> GVALGATRVIYPAGQKQVQLAVTNNDENSTYLIQSWVENADGVKDGRFIVTPPLFAMKGKKENTLRILDATNNQLPQDRESLFWMNVKAIPSMDKSKLTENTLQLAIISRIKLYYRPAKLALPPDQAAEKLRFRRSANSLTLINPTPYYLTVTELNAGTRVLENALVPPMGESTVKLPSDAGSNITYRTINDYGALTPKMTGVMEHHHHHH;> DLYFNPRFLADDPQAVADLSRFENGQELPPGTYRVDIYLNNGYMATRDVTFNTGDSEQGIVPCLTRAQLASMGLNTASVAGMNLLADDACVPLT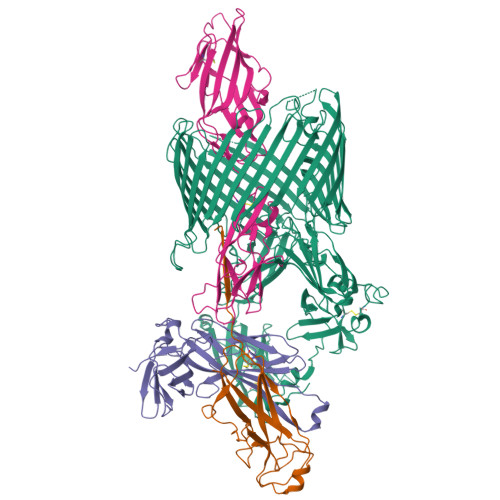TMVQDATAHLDVGQQRLNLTIPQAFMSNRARGYIPPELWDPGINAGLLNYNFSGNSVQNRIGGNSHYAYLNLQSGLNIGAWRLRDNTTWSYNSSDRSSGSKNKWQHINTWLERDIIPLRSRLTLGDGYTQGDIFDGINFRGAQLASDDNMLPDSQRGFAPVIHGIARGTAQVTIKQNGYDIYNSTVPPGPFTINDIYAAGNSGDLQVTIKEADGSTQIFTVPYSSVPLLQREGHTRYSITAGEYRSGNAQQEKPRFFQSTLLHGLPAGWTIYGGTQLADRYRAFNFGIGKNMGALGALSVDMTQANSTLPDDSQHDGQSVRFLYNKSLNESGTNIQLVGYRYSTSGYFNFADTTYSRMNGYNIETQDGVIQVKPKFTDYYNLAYNKRGKLQLTVTQQLGRTSTLYLSGSHQTYWGTSNVDEQFQAGLNTAFEDINWTLSYSLTKNAWQKGRDQMLALNVNIPFSHWLRSDSKSQWRHASASYSMSHDLNGRMTNLAGVYGTLLEDNNLSYSVQTGYAGGGDGNSGSTGYATLNYRGGYGNANIGYSHSDDIKQLYYGVSGGVLAHANGVTLGQPLNDTVVLVKAPGAKDAKVENQTGVRTDWRGYAVLPYATEYRENRVALDTNTLADNVDLDNAVANVVPTRGAIVRAEFKARVGIKLLMTLTHNNKPLPFGAMVTSESSQSSGIVADNGQVYLSGMPLAGKVQVKWGEEENAHCVANYQLPPESQQQLLTQLSAECR;> ADSTITIRGYVRDNGCSVAAESTNFTVDLMENAAKQFNNIGATTPVVPFRILLSPCGNAVSAVKVGFTGVADSHNANLLALENTVSAASGLGIQLLNEQQNQIPLNAPSSALSWTTLTPGKPNTLNFYARLMATQVPVTAGHINATATFTLEYQ;> FACKTANGTAIPIGGGSANVYVNLAPVVNVGQNLVVDLSTQIFCHNDYPETITDYVTLQRGSAYGGVLSNFSGTVKYSGSSYPFPTTSETPRVVYNSRTDKPWPVALYLTPVSSAGGVAIKAGSLIAVLILRQTNNYNSDDFQFVWNIYANNDVVVPTGGCDVSARDVTVTLPDYPGSVPIPLTVYCAKSQNLGYYLSGTTADAGNSIFTNTASFSPAQGVGVQLTRNGTIIPANNTVSLGAVGTSAVSLGLTANYARTGGQVTAGNVQSIIGVTFVYQ> GHMAMEKPVLWYIADPMCSWCWGFAPVIENIRQEYSAFLTVKIMPGGLRPGTNTPLLPEKRAQILHHWHSVHITTGQPFTFENALPEGFIYDTEPACRGVVSVSLIEPEKVFPFFAAIQRAFYVGQEDVAQLAILKKLAVDLGIPESRFTPVFQSDEAKQRTLAGFQRVAQWGISGFPALVVESGTDRYLITTGYRPIEAL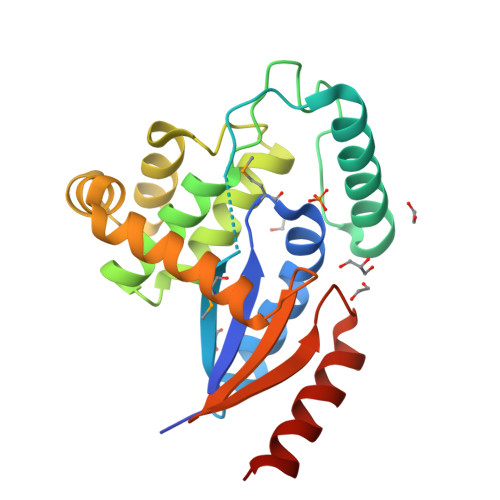RQLLDTWLQQHGVGS> IEPENIGPTF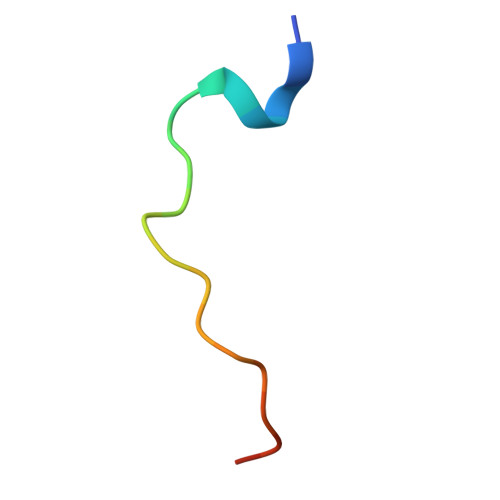SALPPIYIPTG>[2x]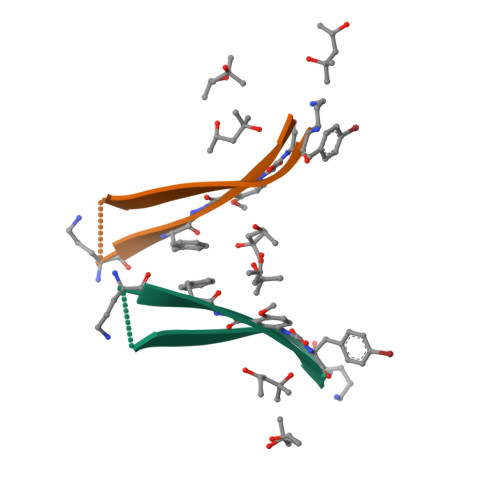AAIIGLMVAKFXYK> GRAMGACSHGPVDVVFLLHATRDNAHNAEAVRRVLERLVSALGPLGPQAAQVGLLTYSHRPSPLFPLNSSHDLGIILRKIRDIPYVDPSGNNLGTAVTTAHRYLLASNAPGRRQQVPGVMVLLVDEPLRGDILSPIREAQTSGLKVMALSLVGADPEQLRRLAPGTDPIQNFFAVDNGPGLDRAVSDLAVALCQAA

Type VII collagen is an extracellular matrix protein, which is important for skin stability. The structure of the vWFA2 subdomain of type VII collagen has been determined, and it has been shown that vWFA2 interacts with integrins.

In addition, a new interaction site for laminin‐332 was identified and characterized. These data provide new insights into vWFA2 functions in the extracellular matrix.> ANGNEGLSTTTKYIFVPIATIGCGKTTVFNTLNNLFPQWTHIQNNNISKKAKLKICDLTLLALEDDDQSVVLFDRNNSASRERRQIFTTIDQKRDEHLDDTVDLKYIAINFIPEDLSEEELWDITYNRVIQRGDNHQSIKSQLDENLVESVMKGFIQRYQPINTSRSPDDQFDHVIHLKLSKDENSLKSSLENVRIIIDDLVQNFPDLIKEKPADELINECFQKALDYKPTFVKNMTANTIKKDPTYYGIAMHYSSILENLEIVSHN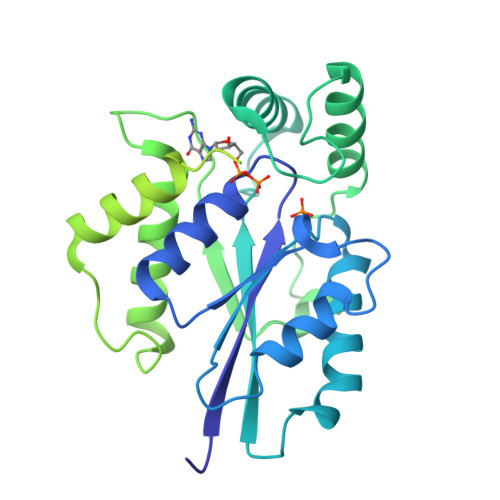EHFQNIKSHIQTEFHVTLGHIASSKQDKAGRVKWKKLVKTLGKGDPNKPKSALKFFADVKLLQIVINTDKLACIKVEILKIYDTNDVLQSEIEPINKQLHITIGCIPPATAVESNITLEELYDNPDEQELKPDGTYKCGDDTLHVFNFDNPDLKLFSQQLFVAYQ>[2x]SPRANEIKKGMVLNYNG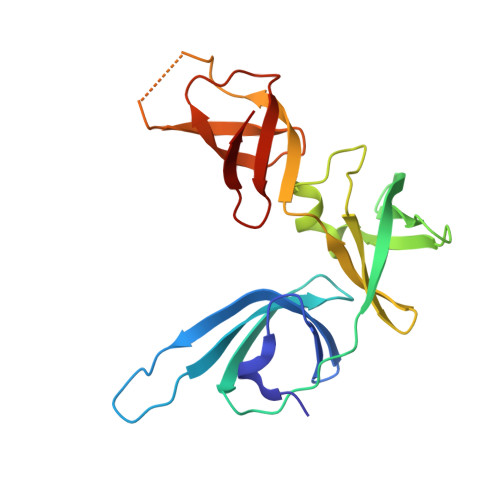KLLLVKDIDIQSPTARGAATLYKMRFSDVRTGLKVEERFKGDDIVDTVTLTRRYVDFSYVDGNEYVFMDKEDYTPYTFTKDQIEEELLFMPEGGMPDMQVLTWDGQLLALELPQTVDLEIVETAPGIKGASASARNKPATLSTGLVIQVPEYLSPGEKIRIHIEERRYMGRAD>[2x]MAHHHHHHMINHPRIGIGILIFNNRNEILLGKRISSHGESSYAPAGGHLEFGETFEECAIREVLEETNLIIEN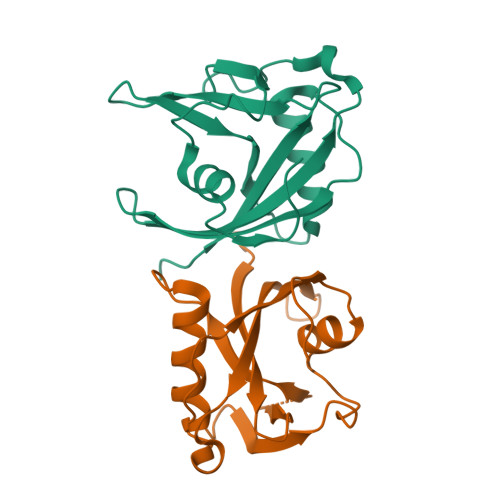PQFIAVTNDIFEKEQKHYVSIFLKAHCLNEHELQNLEPHKVENWQWFALDNLPSNLFLPLKRLIEKKCYLYKEIID N-cyclopropyl-6-[(6,7-dimethoxyquinolin-4-yl)oxy]naphthalene-1-carboxamide 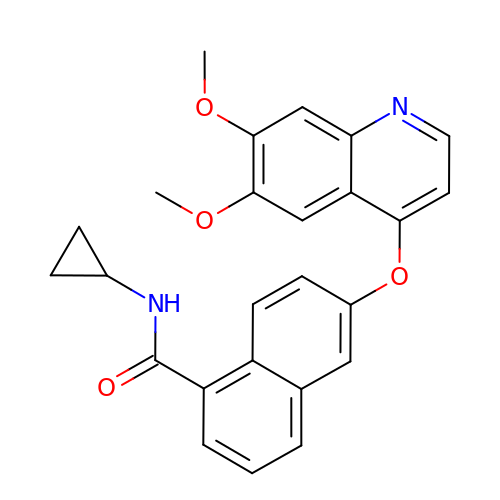| C25 H22 N2 O4 | ZATGFXTWDKIEKC-UHFFFAOYSA-N>MAETPNSDMSGATGGRSKRPKSNQDWWPSKLNLEILDQNARDVGPVEDDFDYAEEFQKLDLEAVKSDLEELMTSSQDWWPADYGHYGPLFIRMAWHSAGTYRTADGRGGAAGGRQRFAPINSWPDNANLDKARRLLLPIKQKYGQKISWADLMILAGNVAIESMGFKTFGYAGGREDAFEEDKAVNWGPEDEFETQERFDEPGEIQEGLGASVMGLIYVNPEGPDGNPDPEASAKNIRQTFDRMAMNDKETAALIAGGHTFGKVHGADDPEENLGPEPEAAPIEQQGLGWQNKNGNSKGGEMITTGIEGPWTQSPTEWDMGYINNLLDYEWEPEKGPGGAWQWAPKSEELKNSVPDAHDPDEKQTPMMLTTDIALKRDPDYREVMETFQENPMEFGMNFAKAWYKLTHRDMGPPERFLGPEVPDEEMIWQDPLPDADYDLIGDEEIAELKEEILDSDLSVSQLVKTAWASASTYRDSDKRGGANGARLRLEPQKNWEVNEPEQLETVLGTLENIQTEFNDSRS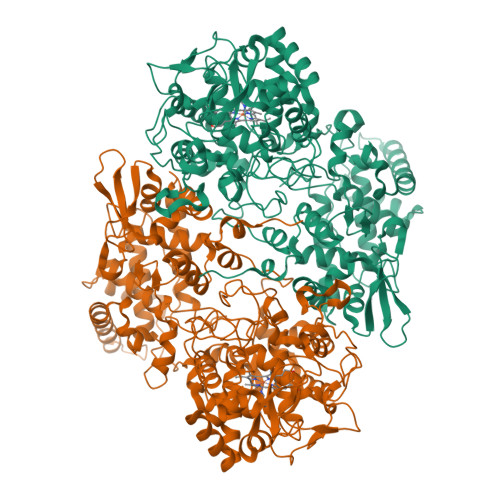DGTQVSLADLIVLGGNAAVEQAAANAGYDVEIPFEPGRVDAGPEHTDAPSFDALKPKVDGVRNYIQDDITRPAEEVLVDNADLLNLTASELTALIGGMRSIGANYQDTDLGVFTDEPETLTNDFFVNLLDMGTEWEPAADSEHRYKGLDRDTGEVKWEATRIDLIFGSNDRLRAISEVYGSADAEKKLVHDFVDTWSKVMKLDRFDLEHHHHHH[2x]> GSAMALK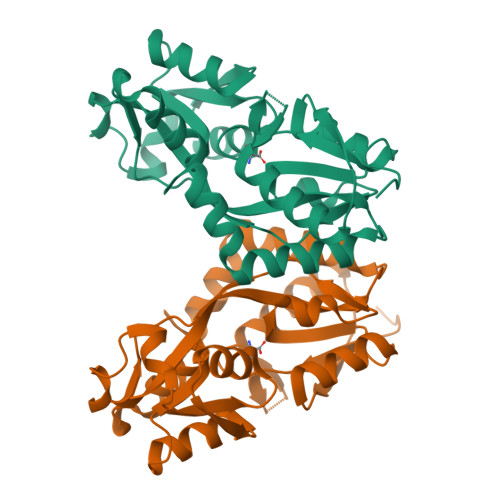VGVVGNPPFVFYGEGKNAAFTGISLDVWRAVAESQKWNSEYVRQNSISAGITAVAEGELDILIGPISVTPERAAIEGITFTQPYFSSGIGLLIPGTATPLFRSVGDLKNKEVAVVRDTTAVDWANFYQADVRETNNLTAAITLLQKKQVEAVMFDRPALIYYTRQNPNLNLEVTEIRVSLEPYGFVLKENSPLQKTINVEMLNLLYSRVIAEFTERWLGPGIEEN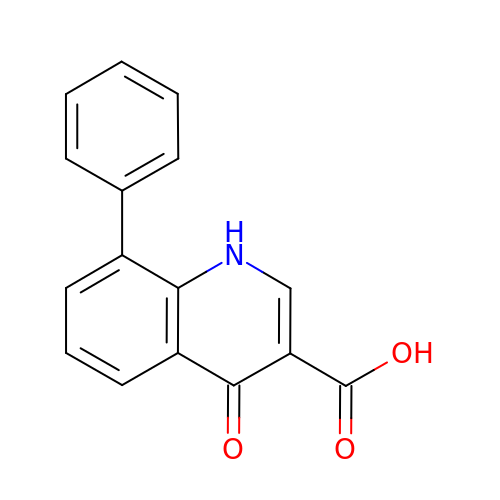4-oxo-8-phenyl-1,4-dihydroquinoline-3-carboxylic acid | C16 H11 N O3 | IYZQCKZKSCOMCY-UHFFFAOYSA-N> MAELQMLLEEEIPGGRRALFDSYTNLERVADYCENNYIQSADKQRALEETKAYTTQSLASVAYLINTLANNVLQMLDIQASQLRRMESSINHISQTVDIHKEKVARREIGILTTN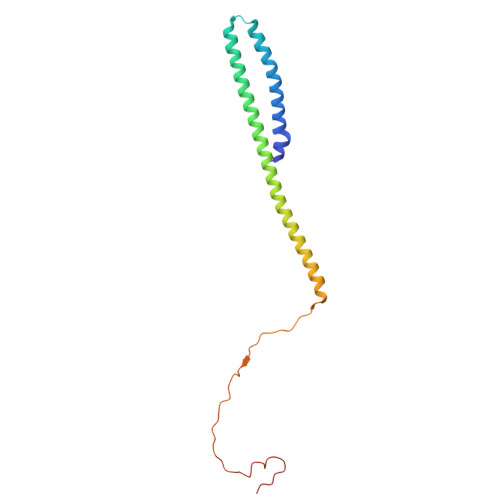KNTSRTHKIIAPANLERPVRYIRKPIDYTILDDIGHGVKVSTQ> GSHMIVQIGRREEFDKKLLGEMHKLRAQVFKERKGWDVSVIDEMEIDGYDALSPYYMLIQEDGQVFG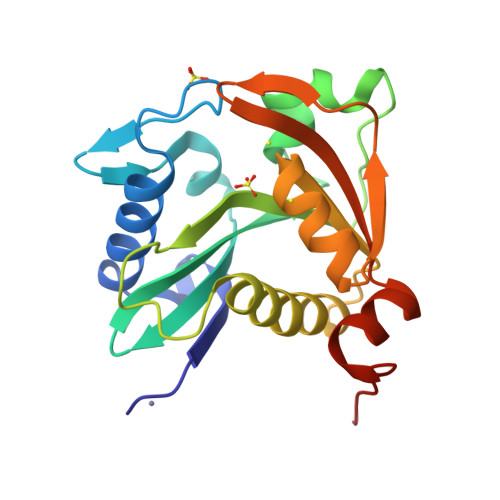CWRILDTTGPYMLKNTFPELLHGKEAPCSPHIWELSRFAINSGQKGSLGFSDCTLEAMRALARYSLQNDIQTLVTVTTVGVEKMMIRAGLDVSRFGPHLKIGIERAVALRIELNAKTQIALYGGVLVEQRLAVS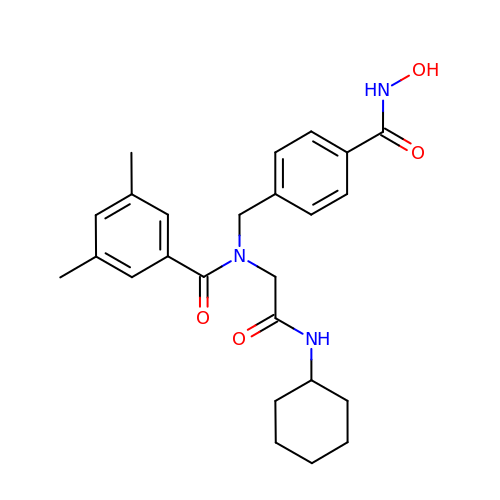N-[2-(cyclohexylamino)-2-oxoethyl]-N-{[4-(hydroxycarbamoyl)phenyl]methyl}-3,5-dimethylbenzamide | C25 H31 N3 O4 | PEXKZGDNGWXGSQ-UHFFFAOYSA-N>GSHMASSCAVQVKLELGHRAQVRKKPTVEGFTHDWMVFVRGPEHSNIQHFVEKVVFHLHESFPRPKRVCKDPPYKVE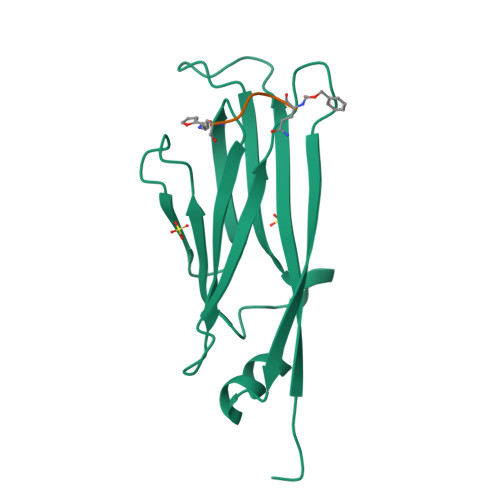ESGYAGFILPIEVYFKNKEEPRKVRFDYDLFLHLEGHPPVNHLRCEKLTFNNPTEDFRRKLLKA[2x]>MNYARFITAASAARNPSPIRTMTDILSRGPKSMISLAGGLPNPNMFPFKTAVITVENGKTIQFGEEMMKRALQYSPSAGIPELLSWLKQLQIKLHNPPTIHYPPSQGQMDLCVTSGSQQGLCKVFEMIINPGDNVLLDEPAYSGTLQSLHPLGCNIINVASDESGIVPDSLRDILSRWKPEDAKNPQKNTPKFLYTVPNGNNPTGNSLTSERKKEIYELARKYDFLIIEDDPYYFLQFNKFRVPTFLSMDVDGRVIRADSFSKIISSGLRIGFLTGPKPLIERVILHIQVSTLHPSTFNQLMISQLLHEWGEEGFMAHVDRVIDFYSNQKDAILAAADKWLTGLAEWHVPAAGMFLWIKVKGINDVKELIEEKAVKMGVLMLPGNAF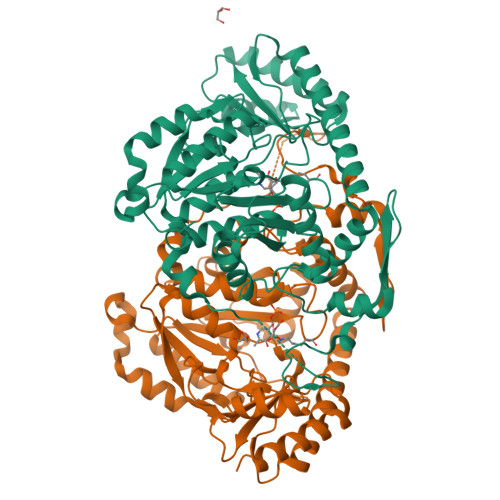YVDSSAPSPYLRASFSSASPEQMDVAFQVLAQLIKESL[4x]>GSHMYLSKQLCFLFYVSSKEIIKKYTNYLKEY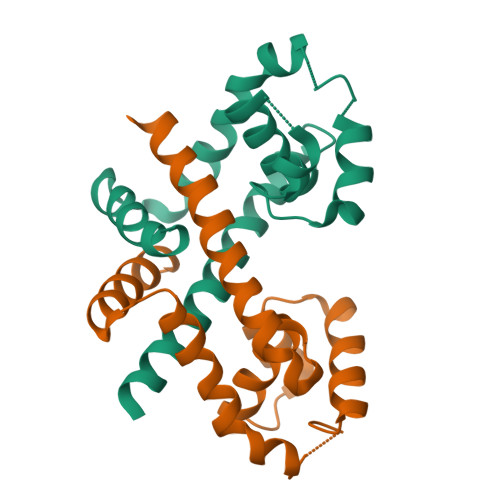DLTYTGYIVLMAIENDEKLNIKKLGERVFLDSGTLTPLLKKLEKKDYVVRTREEKDERNLQISLTEQGKAIKSPLAEISVKVFNEFNISEREASDIINNLRNFVSKNF[2x]> MARQNLKSTDRAVQQMLDKAKREGIQTVWDRYEAMKPQCGFGETGLCCRHCLQGPCRINPFGDEPKVGICGATAEVIVARGLDRSIAAGAAGHSGHAKHLAHTLKKAVQGKAASYMIKDRTKLHSIAKRLGIPTEGQKDEDIALEVAKAALADFHEKDTPVLWVTTVLPPSRVKVLSAHGLIPAGIDHEIAEIMHRTSMGCDADAQNLLLGGLRCSLADLAGCYMGTDLADILFGTPAPVVTESNLGVLKADAVNVAVHGHNPVLSDIIVSVSKEMENEARAAGATGINVVGICCTGNEVLMRHGIPACT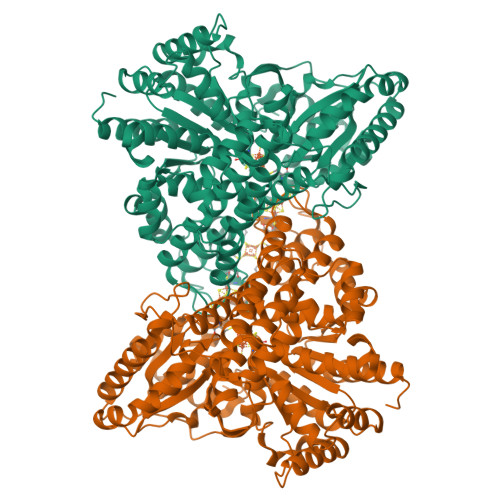HSVSQEMAMITGALDAMILDYQCIQPSVATIAECTGTTVITTMEMSKITGATHVNFAEEAAVENAKQILRLAIDTFKRRKGKPVEIPNIKTKVVAGFSTEAIINALSKLNANDPLKPLIDNVVNGNIRGVCLFAGCNNVKVPQDQNFTTIARKLLKQNVLVVATGCGAGALMRHGFMDPANVDELCGDGLKAVLTAIGEANGLGGPLPPVLHMGSCVDNSRAVALVAALANRLGVDLDRLPVVASAAEAMHEKAVAIGTWAVTIGLPTHIGVLPPITGSLPVTQILTSSVKDITGGYFIVELDPETAADKLLAAINERRAGLGLPW>[2x]MMNKFPGVYKESFTRDYERLHNKISKEVCDQLDDKGYVVIDDCFGHGWASALLEEMRW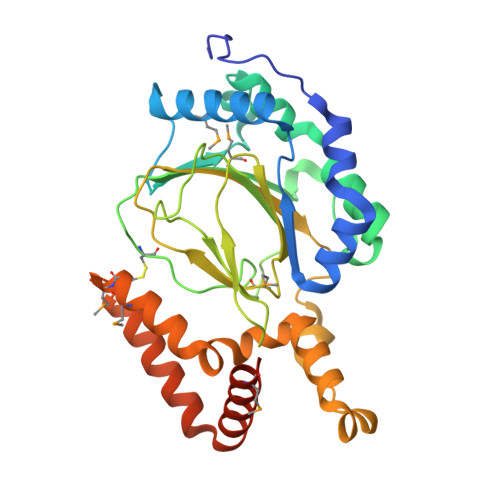LNENDHFKPNKTQFALTQKGSDGKPQAFHFVKPHIFEVDLHDAALRTKVPELDALFHSTELLQALTTHLPQYDLQFSTSDRTLKLQRNAGHGGCFPCHYDNPGAPNKRKVTCLLYLNEGWKEGDGGEVQLFPFLQQPVTVAPKMDRVVLFQSDWMLHRVLPSHAERYVLTIWLDGAKVNAPEDAQLRLTQSDLADWFGFLERLRRSPVQRLLSRGVYEEEYYESLMECMQSTSTEGCVELLKSHETHVENVKRNGPLYGFIQRLRDVRAMNNEEPVHLNLQHHHHHH>[2x]MTEHETKDKAKKIREIYRYDEMSNKVLKVDKRFMNTSQNPQRDAEISQPKSMSGRISAKDMGQGLCNNINKGLKENDVAVEKTGKSASLKKIQQHNTILNSSSDFRLHYYPKDPSNVETYEQILQWVTEVLGNDIPHDLIIGTADIFIRQLKENEENEDGNIEERKEKIQHELGINIDSLKFNELVKLMKNITDYETHPDNSNKQAVAILADDEKSDEEEVTEMSNNANVLGGEINDNEDDDEEYDYNDVEVNSKKKNKRALPNIENDIIKLSDSKTSNIESVPIYSIDEFFLQRKLRSELGYKDTSVIQDLSEKILNDIETLEHNPVALEQKLVDLLKF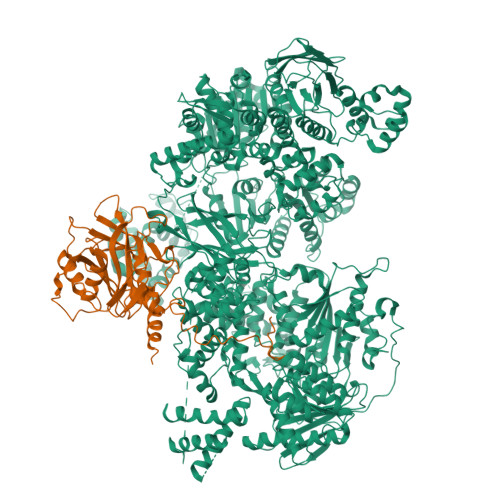ENISLAEFILKNRSTIFWGIRLAKSTENEIPNLIEKMVAKGLNDLVEQYKFRETTHSKRELDSGDDQPQSSEAKRTKFSNPAIPPVIDLEKIKFDESSKLMTVTKVSLPEGSFKRVKPQYDEIHIPAPSKPVIDYELKEITSLPDWCQEAFPSSETTSLNPIQSKVFHAAFEGDSNMLICAPTGSGKTNIALLTVLKALSHHYNPKTKKLNLSAFKIVYIAPLKALVQEQVREFQRRLAFLGIKVAELTGDSRLSRKQIDETQVLVSTPEKWDITTRNSNNLAIVELVRLLIIDEIHLLHDDRGPVLESIVARTFWASKYGQEYPRIIGLSATLPNYEDVGRFLRVPKEGLFYFDSSFRPCPLSQQFCGIKERNSLKKLKAMNDACYEKVLESINEGNQIIVFVHSRKETSRTATWLKNKFAEENITHKLTKNDAGSKQILKTEAANVLDPSLRKLIESGIGTHHAGLTRSDRSLSEDLFADGLLQVLVCTATLAWGVNLPAHTVIIKGTDVYSPEKGSWEQLSPQDVLQMLGRAGRPRYDTFGEGIIITDQSNVQYYLSVLNQQLPIESQFVSKLVDNLNAEVVAGNIKCRNDAVNWLAYTYLYVRMLASPMLYKVPDISSDGQLKKFRESLVHSALCILKEQELVLYDAENDVIEATDLGNIASSFYINHASMDVYNRELDEHTTQIDLFRIFSMSEEFKYVSVRYEEKRELKQLLEKAPIPIREDIDDPLAKVNVLLQSYFSQLKFEGFALNSDIVFIHQNAGRLLRAMFEICLKRGWGHPTRMLLNLCKSATTKMWPTNCPLRQFKTCPVEVIKRLEASTVPWGDYLQLETPAEVGRAIRSEKYGKQVYDLLKRFPKMSVTCNAQPITRSVMRFNIEIIADWIWDMNVHGSLEPFLLMLEDTDGDSILYYDVLFITPDIVGHEFTLSFTYELKQHNQNNLPPNFFLTLISENWWHSEFEIPVSFNGFKLPKKFPPPTPLLENISISTSELGNDDFSEVFEFKTFNKIQSQVFESLYNSNDSVFVGSGKGTGKTAMAELALLNHWRQNKGRAVYINPSGEKIDFLLSDWNKRFSHLAGGKIINKLGNDPSLNLKLLAKSHVLLATPVQFELLSRRWRQRKNIQSLELMIYDDAHEISQGVYGAVYETLISRMIFIATQLEKKIRFVCLSNCLANARDFGEWAGMTKSNIYNFSPSERIEPLEINIQSFKDVEHISFNFSMLQMAFEASAAAAGNRNSSSVFLPSRKDCMEVASAFMKFSKAIEWDMLNVEEEQIVPYIEKLTDGHLRAPLKHGVGILYKGMASNDERIVKRLYEYGAVSVLLISKDCSAFACKTDEVIILGTNLYDGAEHKYMPYTINELLEMVGLASGNDSMAGKVLILTSHNMKAYYKKFLIEPLPTESYLQYIIHDTLNNEIANSIIQSKQDCVDWFTYSYFYRRIHVNPSYYGVRDTSPHGISVFLSNLVETCLNDLVESSFIEIDDTEAEVTAEVNGGDDEATEIISTLSNGLIASHYGVSFFTIQSFVSSLSNTSTLKNMLYVLSTAVEFESVPLRKGDRALLVKLSKRLPLRFPEHTSSGSVSFKVFLLLQAYFSRLELPVDFQNDLKDILEKVVPLINVVVDILSANGYLNATTAMDLAQMLIQGVWDVDNPLRQIPHFNNKILEKCKEINVETVYDIMALEDEERDEILTLTDSQLAQVAAFVNNYPNVELTYSLNNSDSLISGVKQKITIQLTRDVEPENLQVTSEKYPFDKLESWWLVLGEVSKKELYAIKKVTLNKETQQYELEFDTPTSGKHNLTIWCVCDSYLDADKELSFEINVK;>GAMSSKNEWRKSAIANTLLYLRLKNIYVSADDFVEEQNVYVLPKNLLKKFIEISDVKIQVAAFIYGMSAKDHPKVKEIKTVVLVPQLGHVGSVQISNIPDIGDLPDTEGLELLGWIHTQTEELKFMAASEVATHSKLFADKKRDCIDISIFSTPGSVSLSAYNLTDEGYQWGEENKDIMNVLSEGFEPTFSTHAQLLLSDRITGNFIIPSGNVWNYTFMGTAFNQEGDYNFKYGIPLEFYNEMHRPVHFLQFSELAGDEELEAEQIDVFS[2x]trichothecene 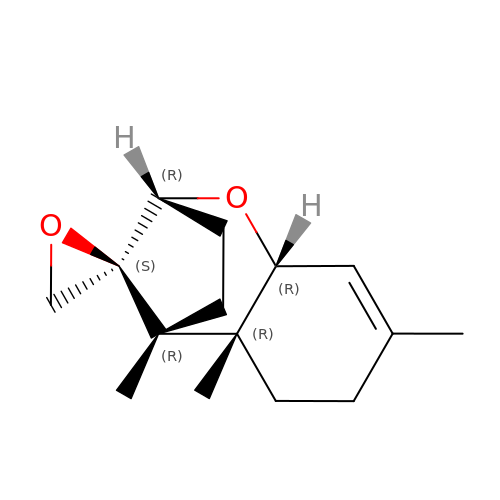| C15 H22 O2 | LZAJKCZTKKKZNT-QMIVOQANSA-N> GTLTGERPPVFWLQGQGCTGCSVTLLNSVHPSIADVLLKVISLEFHPTVMAWEGEHAIEHMRKVAEKFKGKFFLVIEGSVPVEADGKYCIIGEANHHEISMVDALKEFGPNAAAVLAVGT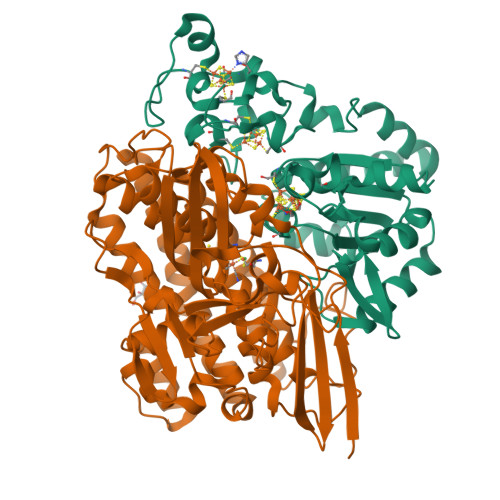CAAYGGIPAAEGSETGATAVSKFLGDNGIKTPVVNIPGCPPHPDWIVGTVVLALDAIKKNGLEGGLAEVVKVLDSDGRPTPFFGRNIHENCPYLDKYDEGVMSATFTDKVGCRYDLGCKGPMTMADCFERKWNGGVNWCVQNAVCIGCVEPDFPDGKSPFYQA;> WSHPQFEKGATGRTTIAIDPVTRIEGHLKAEVVVENGKVVDARLSGGMYRGFETILRGRDPRDASQIVQRICGVCPTAHSTASVLALDEAFGAKVPNNGRITRNLIFGANYLQSHILHFYHLSAQDFVQGPDTAPFVPRFPKSDLRLSKELNKAGVDQYIEALEVRRICHEMVALFGGRMPHVQGQVVGGATEIPTKEKLVEYAARFKKVRDFVEQKYVPVVYTIGSKYKDMFKVGQGFKAALCVGAFPLDNSGKKHLFMPGVYAKGKDMPFDPSKIKEYVKYSWFAEETTGLNYKEGKTIPAPDKAGAYSFVKAPRYDGLSLEVGPLARMWVNNPELSPVGKKLLKDLFGISAKKFRDLGEEAAFSLMGRHVARAEETYYMLGAIEGWLKEIKAGEDTVVMPAVPASAEGTGFTEAPRGSLLHYVKVKDSKIDNYQIVSASLWNCNPRDDMGQRGAVEEALIGIPVDDIQNPVNVARLIRAFDPULACAVH>[2x]SNAIYGYVEKATLIDQNLTLSAKLDTGAKSASLHAVNITEIEKKGIPYLRFTVPTKTGDYSFEGEYVGKVKIKVRSSETNPGLLRTTPIKRPV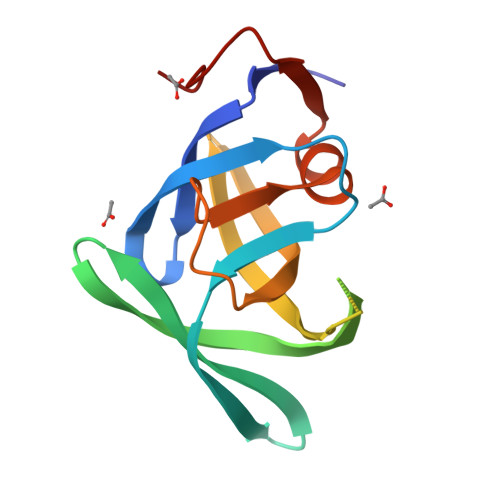VLLNIKLGDKVRTIKVNLTNRKRFLYPLLLGRDAIIDFNGAVDPALTFTTKSK>[2x]SNAGGSSPITGLVYDQRMMLHHNMWDSHHPELPQRISRIFSRHEE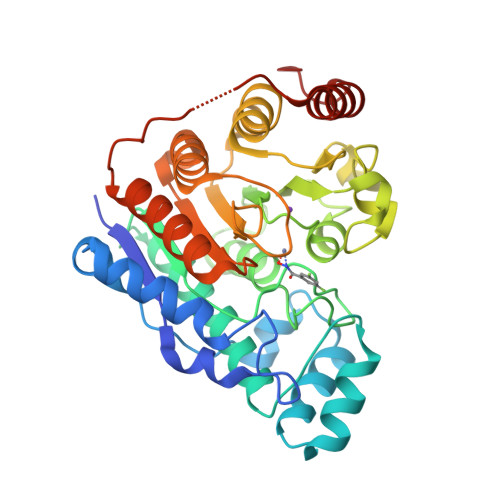LRLLSRCHRIPARLATEEELALCHSSKHISIIKSSEHMKPRDLNRLGDEYNSIFISNESYTCALLAAGSCFNSAQAILTGQVRNAVAIVRPPGHHAEKDTACGFCFFNTAALTARYAQSITRESLRVLIVDWDVHHGNGTQHIFEEDDSVLYISLHRYEDGAFFPNSEDANYDKVGLGKGRGYNVNIPWNGGKMGDPEYMAAFHHLVMPIAREFAPELVLVSAGFDAARGDPLGGFQVTPEGYAHLTHQLMSLAAGRVLIILEGGYNLTSISESMSMCTSMLLGDSPPSLDHLTPLKTSATVSINNVLRAHAPFWSSLR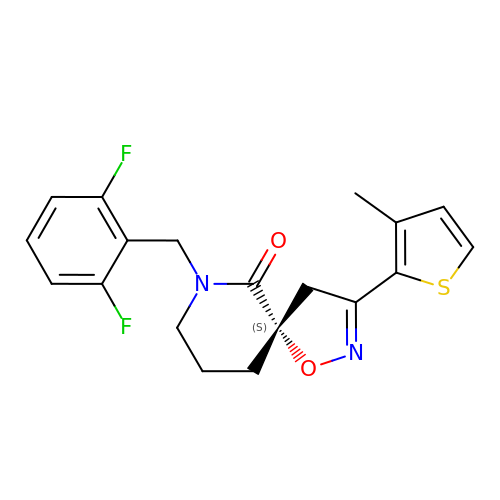(5~{S})-9-[[2,6-bis(fluoranyl)phenyl]methyl]-3-(3-methylthiophen-2-yl)-1-oxa-2,9-diazaspiro[4.5]dec-2-en-10-one | C19 H18 F2 N2 O2 S | GPXGFQYVEMPROU-IBGZPJMESA-N> MSNIQNMSLEDIMGERFGRYSKYIIQDRALPDIRDGLKPVQRRILYSMNKDSNTFDKSYRKSAKSVGNIMGNFHPHGDSSIYDAMVRMSQNWKNREILVEMHGNNGSMDGDPPAAMRYTEARLSEIAGYLLQDIEKKTVPFAWNFDDTEKEPTVLPAAFPNLLVNGSTGISAGYATDIPPHNLAEVIDAAVYMIDHPTAKIDKLMEFLPGPDFPTGAIIQGRDEIKKAYETGKGRVVVRSKTEIEKLKGGKEQIVITEIPYEINKANLVKKIDDVRVNNKVAGIAEVRDESDRDGLRIAIELKKDANTELVLNYLFKYTDLQINYNFNMVAIDNFTPRQVGIVPILSSYIAHRREVILARSRFDKEKAEKRLHIVEGLIRVISILDEVIALIRASENKADAKENLKVSYDFTEEQAEAIVTLQLYRLTNTDVVVLQEEEAELREKIAMLAAIIGDERTMYNLMKKELREVKKKFATPRLSSLEDTAKALEHHHHHH;> MGHHHHHHHHHHSSGHIDDDDKHMSKKEININNYNDDAIQVLEGLDAVRKRPGMYIGSTDGAGLHHLVWEIVDNAVDEALSGFGDRIDVTINKDGSLTVQDHGRGMPTGMHAMGIPTVEVIFTILHAGGKFGQGGYKTSGGLHGVGSSVVNALSSWLEVEITRDGAVYKQRFENGGKPVTTLKKIGTAPKSKTGTKVTFMPDATIFSTTDFKYNTISERLNESAFLLKNVTLSLTDKRTDEAIEFHYENGVQDFVSYLNEDKEILTPVLYFEGEDNGFQVEVALQYNDGFSDNILSFVNNVRTKDGGTHETGLKSAITKVMNDYARKTGLLKEKDKNLEGSDYREGLAAVLSILVPEEHLQFEGQTKDKLGSPLARPVVDGIVADKLTFFLMENGELASNLIRKAIKARDAREAARKARDESRNGKKNKKDKGLLSGKLTPAQSKNPAKNELYLVEGDSAGGSAKQGRDRKFQAILPLRGKVINTAKAKMADILKNEEINTMIYTIGAGVGADFSIEDANYDKIIIMTDADTDGAHIQTLLLTFFYRYMRPLVEAGHVYIALPPLY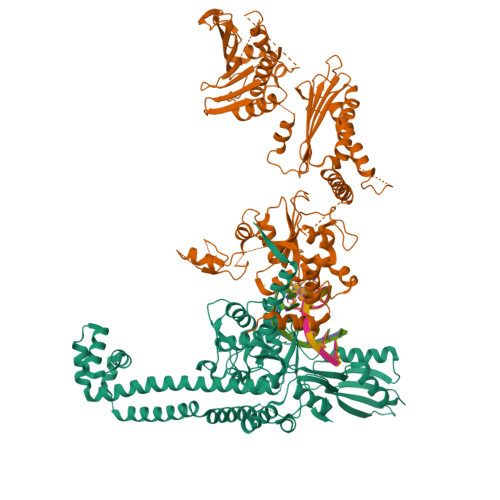KMSKGKGKKEEVAYAWTDGELEELRKQFGKGATLQRYKGLGEMNADQLWETTMNPETRTLIRVTIEDLARAERRVNVLMGDKVEPRRKWIEDNVKFTLEEATVF> GTSTQTKAGSLTIVGTGIESIGQMTLQALSYIEAAAKVFYCVIDPATEAFILTKNKNCVDLYQYYDNGKSRLNTYTQMSELMVREVRKGLDVVGVFYGHPGVFVNPSHRALAIAKSEGYRARMLPGVSAEDCLFADLCIDPSNPGCLTYEASDFLIRDRPVSIHSHLVLFQVGCVGIADFNFTGFDNNKFGVLVDRLEQEYGAEHPVVHYIAAMMPHQDPVTDKYTVAQLREPEIAK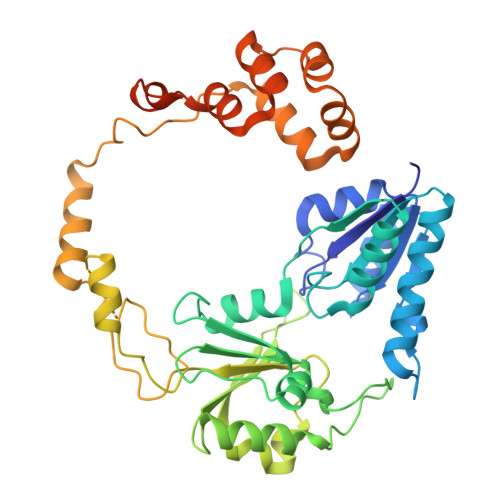RVGGVSTFYIPPKARKASNLDIIRRLELLPAGQVPDKKARIYPANQWEPDVPEVEPYRPSDQAAIAQLADHAPPEQYQPLATSKAMSDVMTKLALDPKALADYKADHRAFAQSVPDLTPQERAALELGDSWAIRCAMKNMPSSLLDAARESGEEASQNGFPWVIVVGVPGVIGSVMSTE> MAFVELLRSAPKRTLSDLLRKLPNHGVGAIVTRDTWHPESKKYWEVVEVAPSTADPTKLSAWGYQYFKGERQHPAPKRIASVWKYGWLLKEQPGAG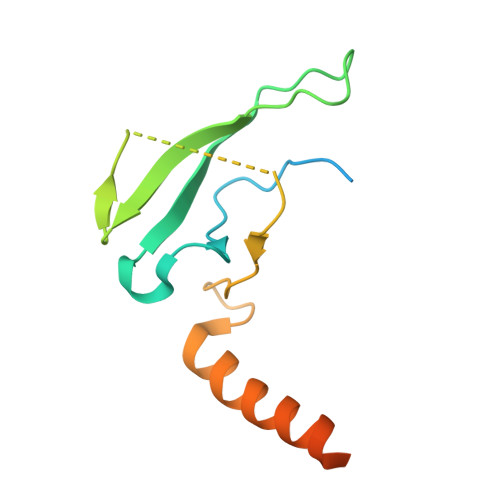LSAAVLQQLSERQAAAQAAGLVAGGSEAAAGTGAAST>SNANDVEEYDAFYKDEINCEVLSWNEQNPKASEERVVGYSLPSVNLQQISNQQLKFASLFKEEPSFAAGVVEMPAGAEKPVKPSKHNIMSFCILQGKIEVTVNATTFRMKKDGVFIVPRGNYYSIKNIGKE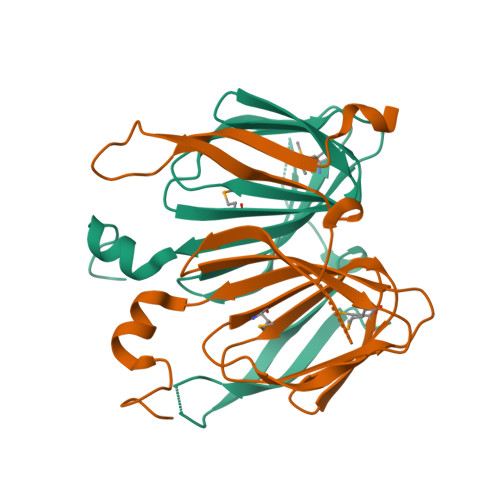AVRLYYTHATDTLENKRRGIGDFPNER[2x]>MWLRLGPPSLSLSPKPTVGRSLCLTLWFLSLALRASTQAPAPTVNTHFGKLRGARVPLPSEILGPVDQYLGVPYAAPPIGEKRFLPPEPPPSWSGIRNATHFPPVCPQNIHTAVPEVMLPVWFTANLDIVATYIQEPNEDCLYLNVYVPTEDVKRISKECARKPNKKICRKGGSGAKKQGEDLADNDGDEDEDIRDSGAKPVMVYIHGGSYMEGTGNMIDGSILASYGNVIVITLNYRVGVLGFLSTGDQAAKGNYGLLDQIQALRWVSENIAFFGGDPRRITVFGSGIGASCVSLLTLSHHSEGLFQRAIIQSGSALSSWAVNYQPVKYTSLLADKVGCNVLDTVDMVDCLRQKSAKELVEQDIQPARYHVAFGPVIDGDVIPDDPEILMEQGEFLNYDIMLGVNQGEGLKFVEGVVDPEDGVSGTDFDYSVSNFVDNLYGYPEGKDTLRETIKFMYTDWADRDNPETRRKTLVALFTDHQWVEPSVVTADLHARYGSPTYFYAFYHHCQSLMKPAWSDAAHGDEVPYVFGVPMVGPTDLFPCNFSKNDVMLSAVVMTYWTNFAKTGDPNKPVPQDTKFIHTKANRFEEVAWSKYNPRDQLYLHIGLKPRVRDHYRATKVAFWKHLVPHLYNLHDMFHYTSTTTKVPPPDTTHSSHITRRPNGKTWSTKRPAISPAYSNENAQGSWNGDQDAGPLLVENPRDYSTELSVTIAVGASLLFLNVLAFAALYYRKDKRRQEPLRQPSPQRGAGAPELGAAPEEELAALQLGPTHHECEAGPPHDTLRLTALPDYTLTLRRSPDDIPLMTPNTITMIPNSLVGLQTLHPYNTFAAGFNSTGLPHSHSTTRV[2x]

Neuroligins are postsynaptic membrane cell adhesion molecules that connect presynaptic and postsynaptic neurons, mediate the transmission of signals between synapses, and shape the characteristics of neural networks through specific synaptic functions. NLGNs belong to single transmembrane proteins, and they all consist of a large extracellular, acetylcholinesterase-like domain (CLD) and a carbohydrate-binding region, following the transmembrane region of O-glycosylation helix and the C-terminal intracellular region as postsynaptic density zone (PDZ) recognition component, which mainly binds to postsynaptic target proteins such as Gephyrin and postsynaptic density protein, thus promoting synaptic differentiation and strengthening the stability of synaptic space and the function of transmitting intersynaptic signals. The ectodomains of NLGNs can form specific cross-synaptic connections with neurexins (NRXNs) of the presynaptic membrane, and these connections can be regulated by the membrane-associated mucin (MAM) domain-containing glycosylphosphatidylinositol anchor (MDGAs). The NLGN structures were highly conserved in both human NLGN2 and human NLGN3 dimer forms as two symmetrical elliptical spheres, and the interface comprises a four-helix bundle including two helices from each protomer.

Although the NLGN3 was used at full length, the size-exclusion chromatography and SDS-PAGE analysis showed that the molecular weight of NLGN3 was similar to NLGN2 ectodomain, with NLGN3 slightly earlier than NLGN2. As the C-terminal flag tag was used for purification and NLGN3 can be purified successfully, it is possible that the C-terminal of NLGN3 was too flexible to be seen in our case. For modeled human NLGN3 dimer, the protomer consists of an α/β hydrolase fold, a 14-stranded central curved β-sheet surrounded by 25 α-helices. The interface area is about 789 Å2, contributed by interface residues including H615, T619, F623, L627, W461, A462, F456, and A622. The overall structure of NLGN2 and NLGN3 protomers is very similar, with root-mean-square deviation (RMSD) of 1.518 Å over 522 Cα atoms. However, when chain A from NLGN2 and NLGN3 was superimposed, the orientation of chain B from NLGN3 has a rotation relative to that from NLGN2, indicating the distinct arrangement adopted by different NLGNs. The interacting residues were mapped to the previously identified patches A–C. The results intuitively showed a slight difference in patch B, where F408 of NLGN2 was substituted by Y431 in NLGN3. The single mutation R451C of NLGN3 is the first single-nucleotide polymorphism associated with ASD. Among them, R451C is a well-known mutation that is closely related to the development of ASD and has recently been found to enhance the gain of function in excitatory synaptic transmission. This residue locates in the central helix of NLGN3, and the mutation may affect the intracellular traffic and membrane localization of NLGN3.> RLVDTDGKPIENDGAEYY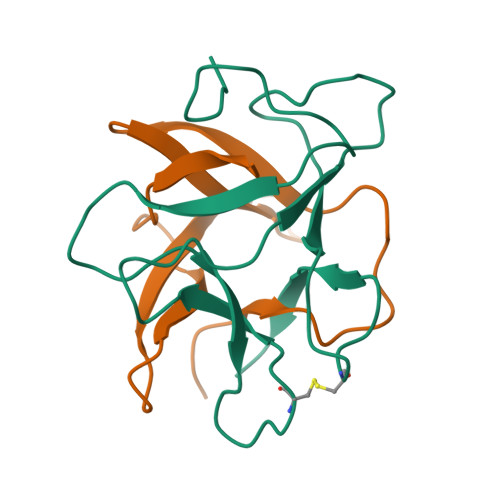ILPSVRGKGGGLVLAKSGGEKCPLSVVQSPSELSNGLPVRFKASPRSKYISVGMLLGIEVIESPECAPKPSMWSVKSG;> WKLPSVTVGNPKVSVFGGPFKIEEGKSGYKDVYSSSKGRDLDDGIEVNKKKEKRLVVKDGNPFIIRFKKSG>MKSSHHHHHHENLYFQSNAETIEIIKDLFEHLCGVRVHRTYEDDTGLWFDTSQGSKNGIMDYKLGFVKSQAENTTEVDTEVIYVPLLKQRTAEELQELQKKLPDYLFETLSFPLRSLNQFYIKMSKSLNKKV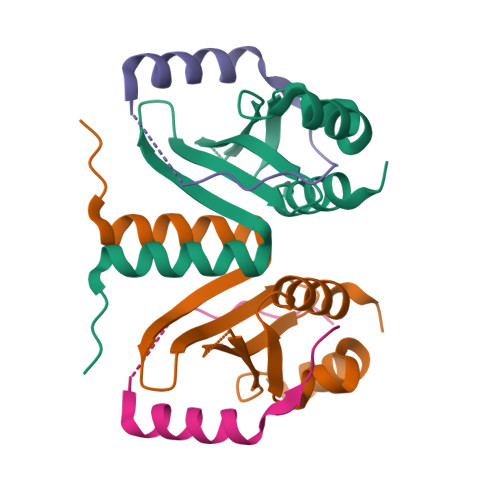[4x];>[4x]DLKFKRHKNKHIQGFPTLGERLDNLQDIKKAKRVENFNSS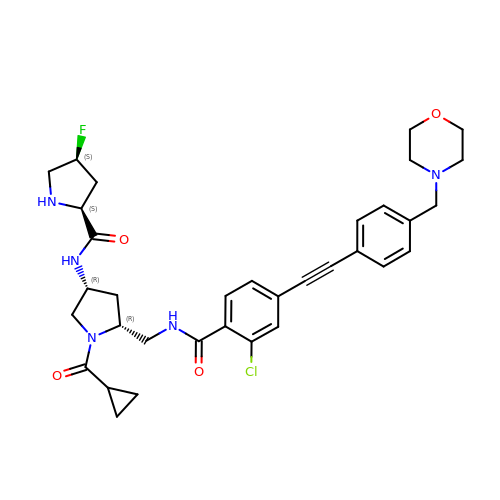(2S,4S)-N-((3R,5R)-5-((2-chloro-4-((4-(morpholinomethyl)phenyl)ethynyl)benzamido)methyl)-1-(cyclopropanecarbonyl)pyrrolidin-3-yl)-4-fluoropyrrolidine-2-carboxamide | C34 H39 Cl F N5 O4 | GIGCGLXLMRWTTB-INXMUBLWSA-N>AHNNENVSGISAYLLGLIIGDGGLYKLKYKGNRSEYRVVITQKSENLIKQHIAPLMQFLIDELNVKSKIQIV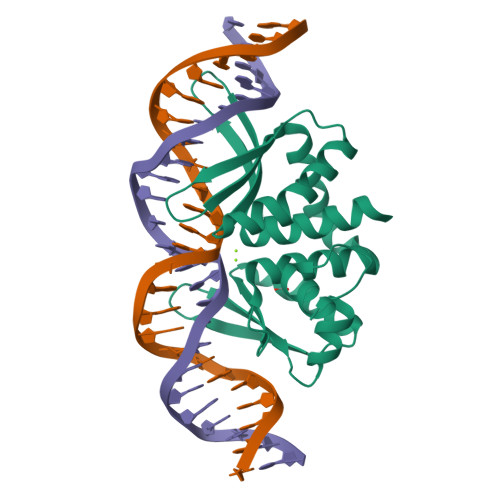KGDTRYELRVSSKKLYYYFANMLERIRLFNMREQIAFIKGLYVAEGDKTLKRLRIWNKNKALLEIVSRWLNNLGVRNTIHLDDHRHGVYVLNISLRDRIKFVHTILSSHLNPLPPEAAALEHHHHHH[3x]> GLGYGSWEIDPKDLTFLKELGTGQFGVVKYGKWRGQYDVAIKMIKEGSM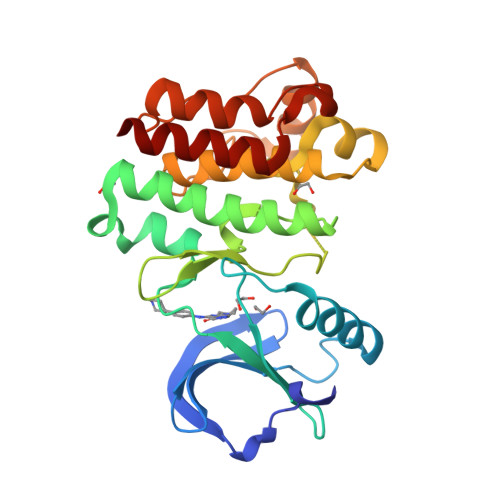SEDEFIEEAKVMMNLSHEKLVQLYGVCTKQRPIFIITEYMANGCLLNYLREMRHRFQTQQLLEMCKDVCEAMEYLESKQFLHRDLAARNCWVNDQGVVKVSDFGLSRYVLDDEYTSSVGSKFPVRWSPPEVLMYSKFSSKSDIWAFGVLMWEIYSLGKMPYERFTNSETAEHIAQGLRLYRPHLASEKVYTIMYSCWHEKADERPTFKILLSNILDVMDEE>SGGSTWQWVLINISEEARQRIEEYVRRISKKEGTEVHFEKDDGVLHIRVKNLHEKRAREIHEYA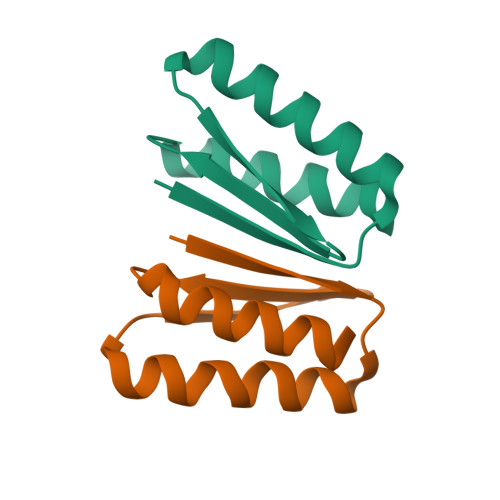KRVIL[2x];>[2x]SGGSSSIFLLSNVSEEARQRAEEYVRRISKKEGTEVRFEKDDGFLTIEVKNLSEERLREIAEYLWRVAV> MGKITFYEDRGFQGHCYECSSDCPNLQPYF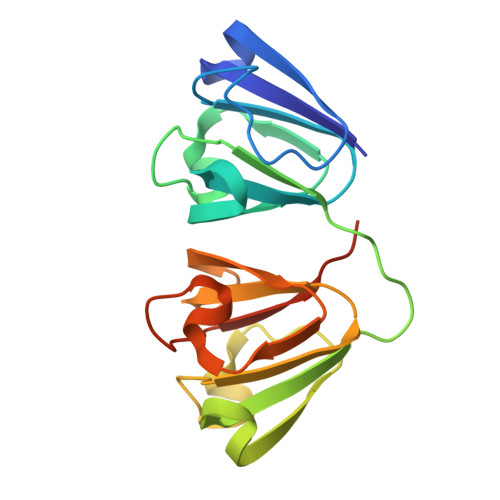SRCNSIRVDSGCWMLYERPNYQGHQYFLRRGDYPDYQQWMGFNDSIRSCRLIPQHTGTFRMRIYERDDFRGQMSEITDDCPSLQDRFHLTEVHSLNVLEGSWVLYEMPSYRGRQYLLRPGEYRRYLDWGAMNAKVGSLRRVMDFYHHHHHH> 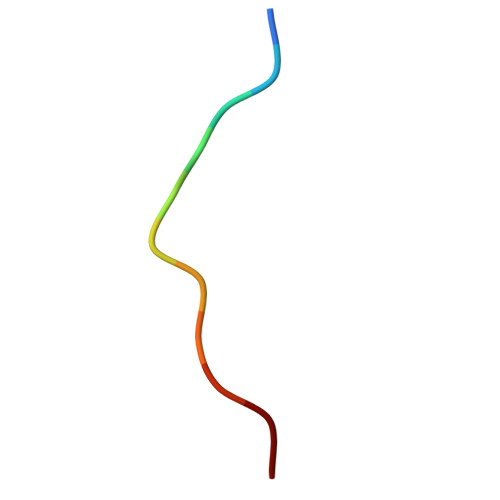GPVFTSRSAAG> MFDPA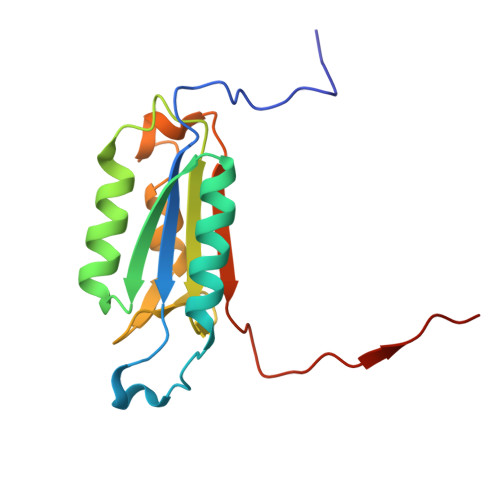EKYKMDHRRRGIALIFNHERFFWHLTLPERRGTCADRDNLTRRFSDLGFEVKCFNDLKAEELLLKIHEVSTVSHADADCFVCVFLSHGEGNHIYAYDAKIEIQTLTGLFKGDKCHSLVGKPKIFIIQACRGNQHDVPVIPLDVVD> SGSGSG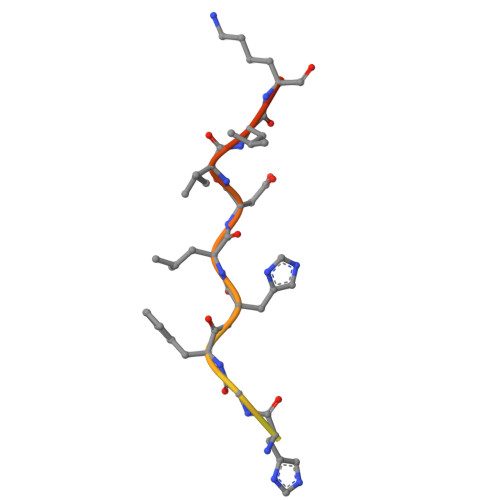SGSGSEFNHGFHLDILKGRK> MSLSFMIGYSWTQTEPGQVNHILDQFLSSMVREAGAVNYFVLPFPFSEDRSQI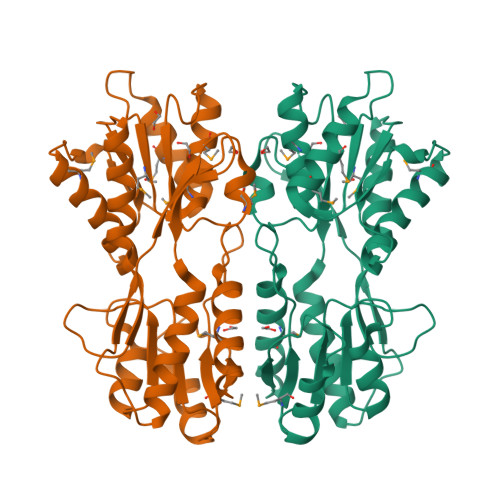DIYRDLIRSGNVDGFVLSSINYNDPRVQFLLKQKFPFVAFGRSNPDWDFAWVDIDGTAGTRQAVEYLIGRGHRRIAILAWPEDSRVGNDRLQGYLEAMQTAQLPIETGYILRGEGTFEVGRAMTLHLLDLSPERRPTAIMTLNDTMAIGAMAAARERGLTIGTDLAIIGFDDAPMVQYLFPPLSSVRQPIAEAGRKCIELLVAIVEGREPEQKHILLQPSLIIRASEGHHHHHH>GSQSGPLPKPSLQA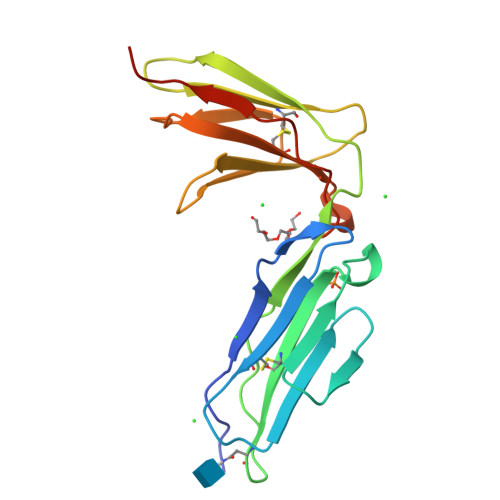LPSSLVPLEKPVTLRCQGPPGVDLYRLEKLSSSRYQDQAVLFIPAMKRSLAGRYRCSYQNGSLWSLPSDQLELVATGVFAKPSLSAQPGSGGDVTLQCQTRYGFDQFALYKEGDPERWYRASFPIITVTAAHSGTYRCYSFSSRDPYLWSAPSDPLELVVTGTSAAA[4x]>RTEDLPKAVVFLEPQWYRVLEKDSVTLKCQGAYSPEDNSTQWFHNESLISSQASSYFIDAATVDDSGEYRCQTNLSTLSDPVQLEVHIGWLLLQAPRWVFKEEDPIHLRCHSWKNTALHKV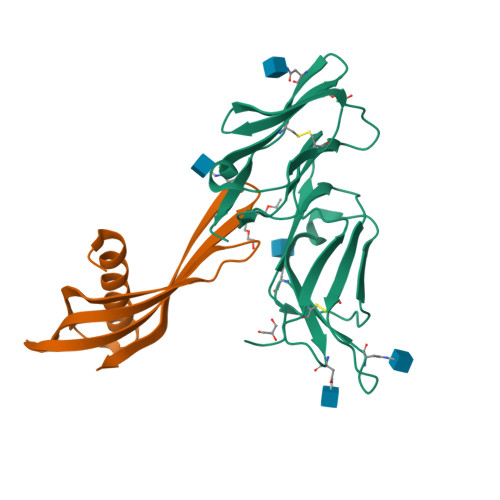TYLQNGKGRKYFHHNSDFYIPKATLKDSGSYFCRGLFGSKNVSSETVNITITQG[2x];>[2x]ATGVRAVPGNENSLEIEELARFAVDEHNKKENALLEFVRVVKAKEQAMNTGFTLATMYYLTLEAKDGGKKKLYEAKVWVKNTQWHNAMTNFKELQEFKPVG>MENTENSVDSKSIKNLEPKIIHGSESMDSGISLDNSYKMDYPEMGLCIIINNKNFHKSTGMTSRSGTDVDAANLRETFRNLKYEVRNKNDLTREEIVELMRDVSKEDHSKRSSF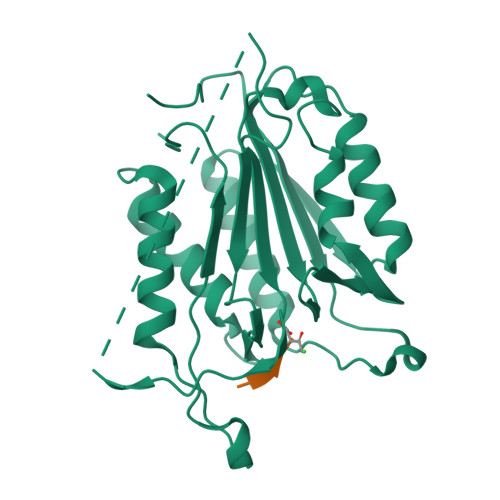VCVLLSHGEEGIIFGTNGPVDLKKITNFFRGDRCRSLTGKPKLFIIQACRGTELDCGIETDSGVDDDMACHKIPVEADFLYAYSTAPGYYSWRNSKDGSWFIQSLCAMLKQYADKLEFMHILTRVNRKVATEFESFSFDATFHAKKQIPCIHSMLTKELYFYH[2x]>[2x]MGSSHHHHHHSQDPMMEYKIVENGLTYRIGNGASVPISNTGELIKGLRNYGPYEVPSLKYNQIALIHNNQFSSLINQLKSQISSKIDEVWHIHNINISEFIYDSPHFDSIKSQVDNAIDTGVDGIMLVLPEYNTPLYYKLKSYLINSIPSQFMRYDILSNRNLTFYVDNLLVQFVSKLGGKPWILNVDPEKG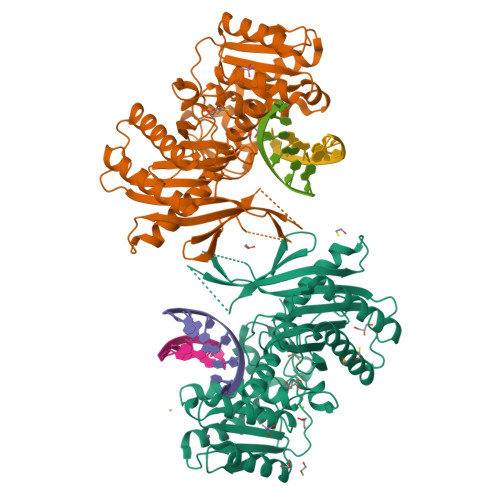SDIIIGTGATRIDNVNLFCFAMVFKKDGTMLWNEISPIVTSSEYLTYLKSTIKKVVYGFKKSNPDWDVEKLTLHVSGKRPKMKDGETKILKETVEELKKQEMVSRDVKYAILHLNETHPFWVMGDPNNRFHPYEGTKVKLSSKRYLLTLLQPYLKRNGLEMVTPIKPLSVEIVSDNWTSEEYYHNVHEILDEIYYLSKMNWRGFRSRNLPVTVNYPKLVAGIIANVNRYGGYPINPEGNRSLQTNPWFL4-[[(1R,2R)-2-[(3R)-3-azanylpiperidin-1-yl]-2,3-dihydro-1H-inden-1-yl]oxy]-3-chloranyl-benzenecarbonitrile 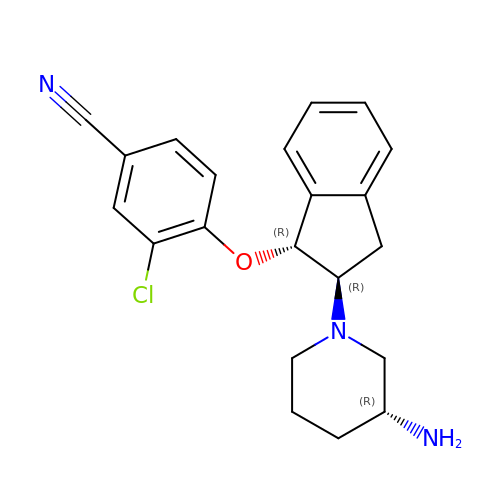| C21 H22 Cl N3 O | RLKRLNQEXBPQGQ-OZOXKJRCSA-N> DMRPEIWIAQEYRRIGDEFNA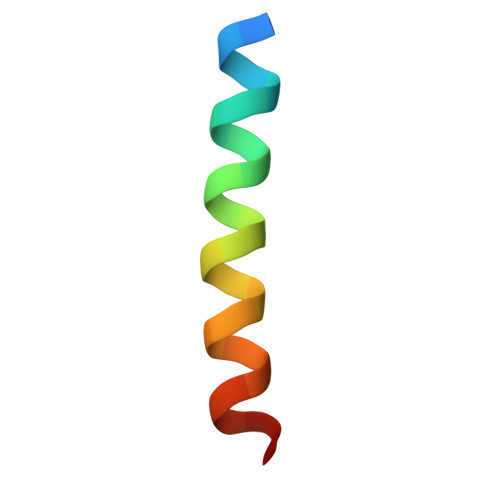YYARR>[2x]GSMTPKYEDLRAYYTKPSFEFEKQFGFMLKPWTTVRFMNVIPNRFIYKIALVGKDEKKYKDGPYDNIDVFIVLEDNKYQ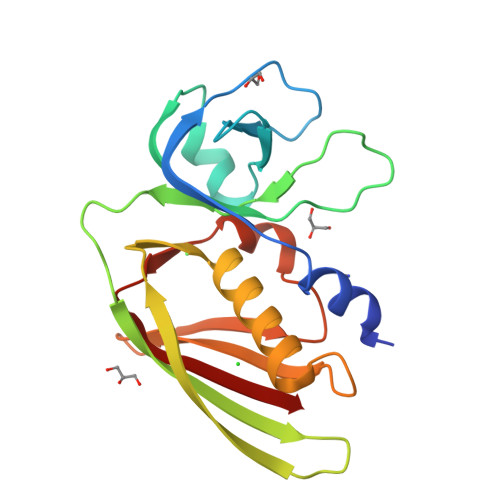LKKYSVGGITKTNSKKVNHKVELSITKKDNQGMISRDVSEYMITKEEISLKELDFKLRKQLIEKHNLYGNMGSGTIVIKMKNGGKYTFELHKKLQEHRMADVIDGTNIDNIEVNIK> NSWGSQMDLTDPLCIEDDTENCKQTMSPNELGLTSAQDDGPLGQEKPNYFLNFRSMNVDIFTVSHTKVDNLFGRAWFFMEHTFTNEGQWRVPLEFPKQGHGSLSLLFAYFTGELNIHVLFLSERGFLRVAHTYDTSNDRVNFLSSNGVITVPAGEQMTLSAPYYSNKPLRTVRDNNSLGYLMCKPFLTGTSTGKIEVYLSLRCPNFFFPLPAPKVTSSRALRGDMANLTNQSPY;> APNGKKKNWKKIMTMSTKYKWTRTKIDIAEGPGSMNMANVLCTTGAQSVALVGERAFYDPRTAGSKSRFDDLVKIAQLFSVMADSTTPSENHGVDAKGYFKWSATTAPQSIVHRNIVYLRLFPNLNVFVNSYSYFRGSLVLRLSVYASTFNRGRLRMGFFPNATTDSTSTLDNAIYTICDIGSDNSFEITIPYSFSTWMRKTNGHPIGLFQIEVLNRLTYNSSSPSEVYCIVQGKMGQDARFFCPTGSVVTFQ;> METIKSIADMATGVVSSVDSTINAVNEKVESVGNEIGGNLLTKVADDASNILGPNCFATTAEPENKNVVQATTTVNTTNLTQHPSAPTMPFSPDFSNVDNFHSMAYDITTGDKNPSKLVRLETHEWTPSWARGYQITHVELPKVFWDHQDK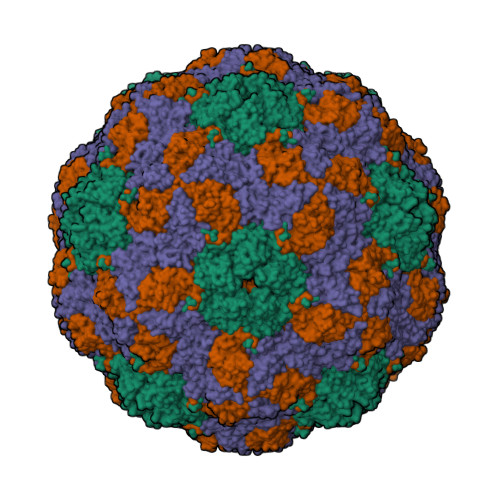PAYGQSRYFAAVRCGFHFQVQVNVNQGTAGSALVVYEPKPVVTYDSKLEFGAFTNLPHVLMNLAETTQADLCIPYVADTNYVKTDSSDLGQLKVYVWTPLSIPTGSANQVDVTILGSLLQLDFQNPRVFAQDVNIYDN> RLYWDDLKRKLSEKLDSTDFTSTIKLLNENSYVPREAGSQKDENLALYVENQFREFKLSKVWRDQHFVKIQVKDSAQNSVIIVDKNGRLVYLVENPGGYVAYSKAATVTGKLVHANFGTKKDFEDLYTPVNGSIVIVRAGKITFAEKVANAESLNAIGVLIYMDQTKFPIVNAELSFFGHAHLGTGDPYTPGFPSFNHTQFPPSRSSGLPNIPVQTISRAAAEKLFGNMEGDCPSDWKTDSTCRMVTSESKNVKLTVSNVLKEIKILNIFGVIKGFVEPDHYVVVGAQRDAWGPGAAKSGVGTALLLKLAQMFSDMVLKDGFQPSRSIIFASWSAGDFGSVGATEWLEGYLSSLHLKAFTYINLDKAVLGTSNFKVSASPLLYTLIEKTMQNVKHPVTGQFLYQDSNWASKVEKLTLDNAAFPFLAYSGIPAVSFCFCEDTDYPYLGTTMDTYKELIERIPELNKVARAAAEVAGQFVIKLTHDVELNLDYERYNSQLLSFVRDLNQYRADIKEMGLS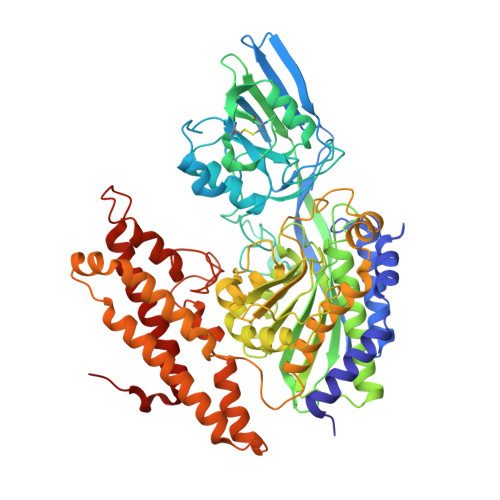LQWLYSARGDFFRATSRLTTDFGNAEKTDRFVMKKLNDRVMRVEYHFLSPYVSPKESPFRHVFWGSGSHTLPALLENLKLRKQNNGAFNETLFRNQLALATWTIQGAANALSGDVWDIDNEF> DPNQAVLKFTTEIHPSCVTRQKVIGAGEFGEVYKGMLKTSSGKKEVPVAIKTLKAGYTEKQRVDFLGEAGIMGQFSHHNIIRLEGVISKYKPMMIITEYMENGALDKFLREKDGEFSVLQLVGMLRGIAAGMKYLANMNYVHRDLAARNILVNSNLVCKVSDFGLSRVLEDDPEATYTTSGGKIPIRWTAPEAISYRKFTSASDVWSFGIVMWEVMTYGERPYWELSNHEVMKAINDGFRLPTPMDCPS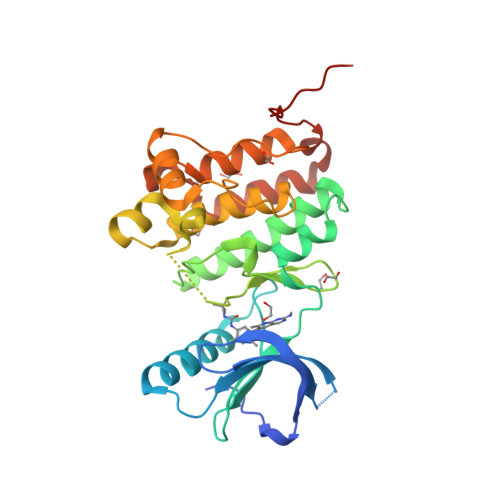AIYQLMMQCWQQERARRPKFADIVSILDKLIRAPDSLKTLADFDPRVSIRLPSTSG> HMQLEIQVALNFIISYLYNKLPRRRVNIFGEELERLLKKKYEGHWYPEKPYKGSGFRCIHIGEKVDPVIEQASKESGLDIDDVRGNLPQDLSVWIDPFEVSYQIGEKGPVKVLYVDDNNENGCELDKEIKNSFNPEAQVFMPISDPASSVSSSPSPPFGHSAAVSPTFMPRSTQPLTFTTATFAATKFGSTKMKNSGRSNKVARTSPINLGLNVNDLLK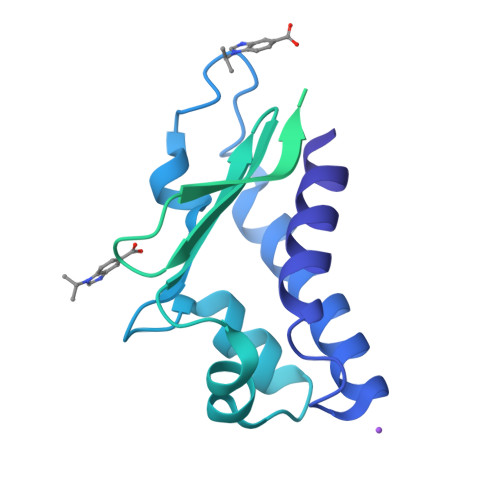QKAISSSMHSLYGLGLGSQQQPQQQQQPAQPPPPPPPPQQQQQQKTSALSPNAKEFIFPNMQGQGSSTNGMFPGDSPLNLSPLQYSNAFDVFAAYGGLNEKSFVDGLNFSLNNMQYSNQQFQPVMAN compound 28 | C22 H26 N4 O2 | 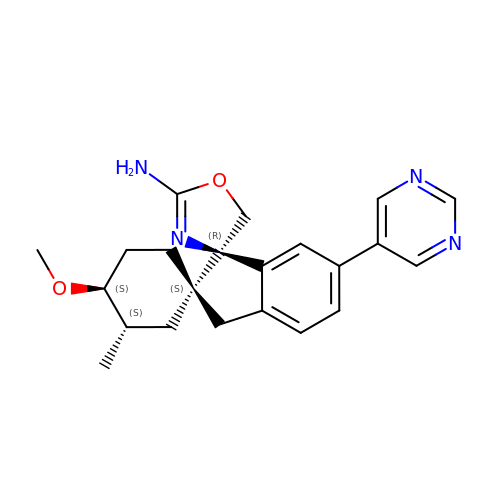LNZBKHMXPFCMOB-GLYDZZHWSA-N1,10-PHENANTHROLINE 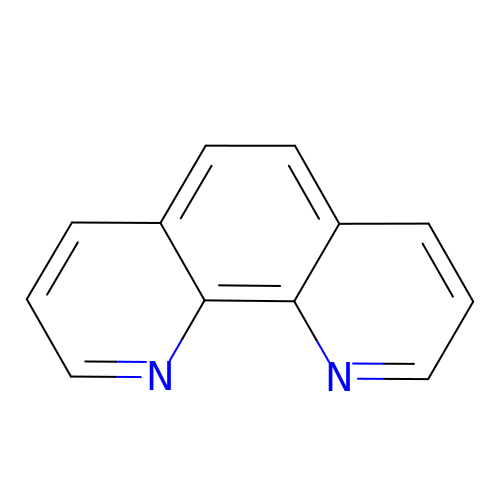| C12 H8 N2 | DGEZNRSVGBDHLK-UHFFFAOYSA-N> MAKRRNRKTRFNLPPGKSGWPFLGETIGYLKPYTATTLGDFMQQHVSKYGKIYRSNLFGEPTIVSADAGLNRFILQNEGRLFECSYPRSIGGILGKWSMLVLVGDMHRDMRSISLNFLSHARLRTILLKDVERHTLFVLDSWQQNSIFSAQDEAKKFTFNLMAKHIMSMDPGEEETEQLKKEYVTFMKGVVSAPLNLPGTAYHKALQSRATILK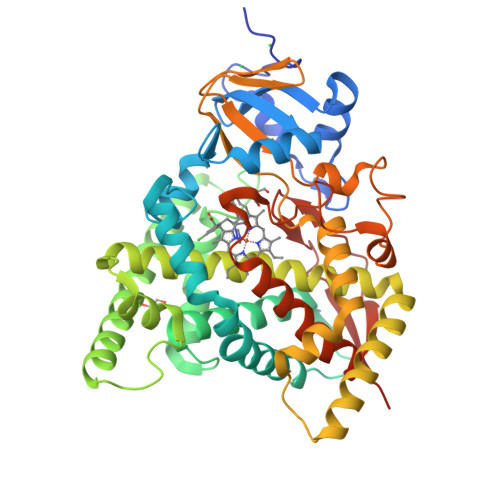FIERKMEERKLDIKERKQRTDDDLLGWVLKHSNLSTEQILDLILSLLFAGHETSSVAIALAIFFLQACPKAVEELREEHLEIARAKKELGESELNWDDYKKMDFTQCVINETLRLGNVVRFLHRKALKDVRYKGYDIPSGWKVLPVISAVHLDNSRYDQPNLFNPWRWQQQNTWGNNYMPFGGGPRLCAGSELAKLEMAVFIHHLVLKFNWELAEDDKPFAFPFVDFPNGLLIRVSRILHHHH> NNEIKPGKMKVKATKG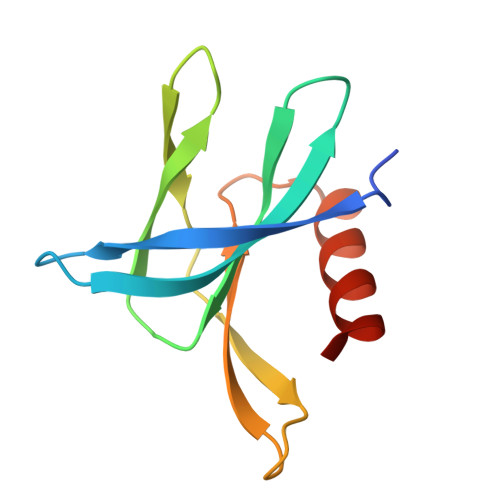EGDGGITSEGNALYNNEGGRAFMYAYVTTKPGMKYVKWEHDSGVVTVELEPPARFVIDTPTGPQIKYLYFVKNLNNLRRGAVLGYIGATVRLQ> MKVGQDKVVTIRYTLQVEGEVLDQGELSYLHGHRNLIP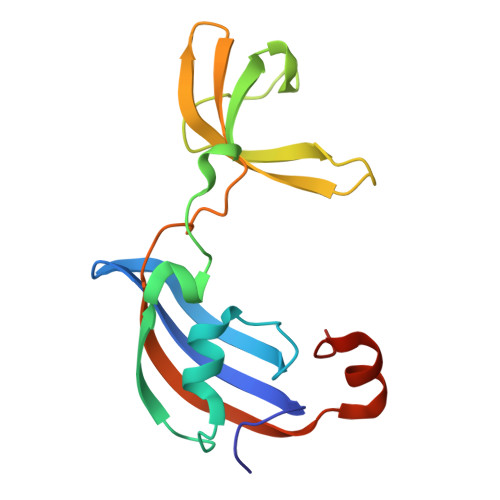GLEEALEGREEGEAFQAHVPAEKAYGPHDPEGVQVVPLSAFPEDAEVVPGAQFYAQDMEGNPMPLTVVAVEGEEVTVDFNHPLAGKDLDFQVEVVKVREATPEELLHGHAHLVPK>GSRKIIHVDMDCFAAAVEMRDNPALRDIPIAIGGSRERRGVISCANYPARKFGVRSAMPTGMALKLCPHLTLLPGRFDAYKEASNHIREIFSRYTSRIEPLSLDEAYLDVTDSVHCHGSATLIAQEIRQTIFNELQLTASAGVAPVKFLAKIASDMNKPNGQFVITPAEVPAFLQTLPLAKIPGVGKVSAAKLEAMGLRTCGDVQKCDLVMLLKRFGKFGRILWERSQGIDERDVNSERLRKSVGVERTMAEDIHHWSECEAIIERLYPELE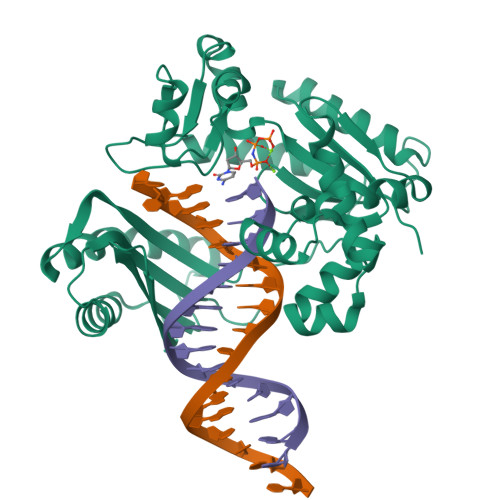RRLAKVKPDLLIARQGVKLKFDDFQQTTQEHVWPRLNKADLIATARKTWDERRGGRGVRLVGLHVTLLDP[2x]octyl 3,4,5-trihydroxybenzoate 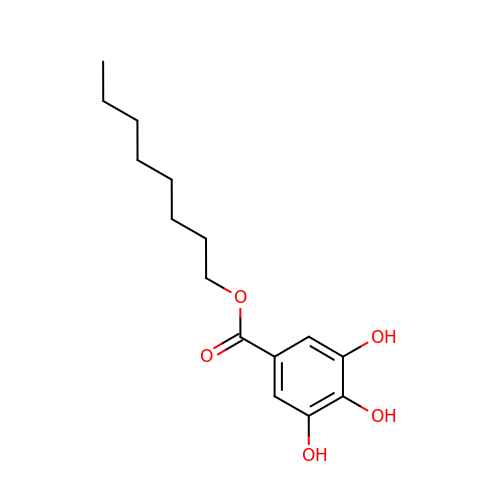| C15 H22 O5 | NRPKURNSADTHLJ-UHFFFAOYSA-N> SKGENSKLNPWAVVGFIDAEGSFMVRVRKNSKYKTGWLVVAIFSVTVDKKDLFLLESLKTFFGGLGSIKKSGNSTFSYRIESSEQLTKIILPFFDKYSLITEKLGDYLLFKKVLELMGTKEHLTQRGLEKIVSLKASINKGLSEELQAAFPQCVPTPRPEINNKNIPDPFWLAGFVSGDGSFKSILKKSESIKVGFQSILVFQIT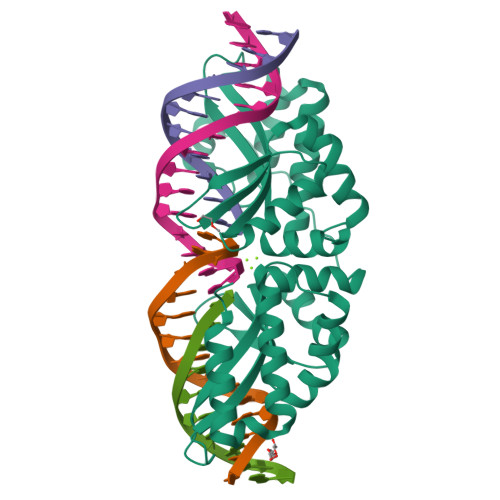QHARDVKLMESLISYLGCGFIEKDSRGPWLYYTVTNFSDIQGKIIPFFHQYKIIGSAYGDYQDWCKIALIMQNKNHLTPEGLNEIRALKGGMNKGRL> MI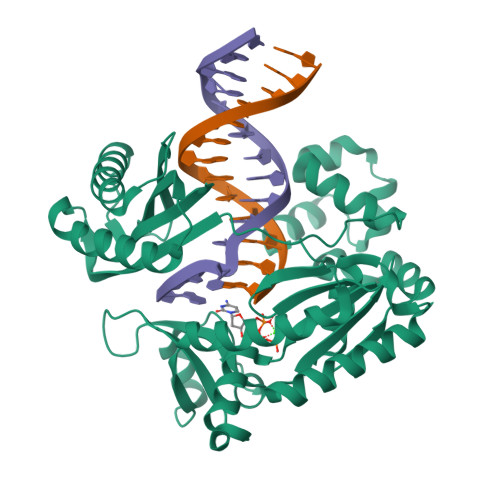VLFVDFDYFYAQVEEVLNPSLKGKPVVVCVFSGRFEDSGAVATANYEARKFGVKAGIPIVEAKKILPNAVYLPMRKEVYQQVSSRIMNLLREYSEKIEIASIDEAYLDISDKVRDYREAYNLGLEIKNKILEKEKITVTVGISKNKVFAKIAADMAKPNGIKVIDDEEVKRLIRELDIADVPGIGNITAEKLKKLGINKLVDTLSIEFDKLKGMIGEAKAKYLISLARDEYNEPIRTRVRKSIGRIVTMKRNSRNLEEIKPYLFRAIEESYYKLDKRIPKAIHVVAVTEDLDIVSRGRTFPHGISKETAYSESVKLLQKILEEDERKIRRIGVRFSKFIEAIGLDKFFDTGGHHHHHH>[8x]SNARYTNILVPVDSSDAAQAAFTEAVNIAQRH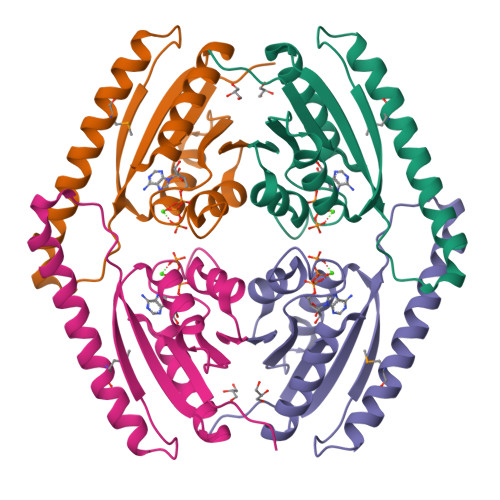QANLTALYVVDDSAYHTPALDPVLSELLDAEAAHAKDAMRQRQQFVATTSAPNLKTEISYGIPKHTIEDYAKQHPEIDLIVLGATGTNSPHRVAVGSTTSYVVDHAPCNVIVIR>[4x]VPEITTAQTIANSVVDAKKFDYLFGKATGNSHTLDRTNQLALEMKRLGVADDINGHAVLAEHFTQATKDSN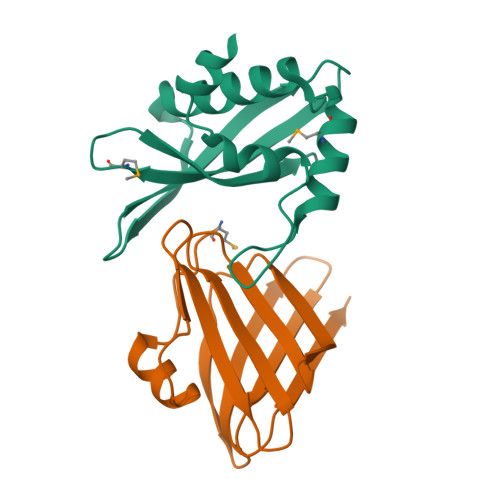NIVKKYTDQYGSFEIRESFFIGPSGKATVFESTFEVMKDGSHRFITTIPKNGVTK;>MFIENKPGEIELLSFFESEPVSFERDNISFLYTAKNKCGLSVDFSFSVVEGWIQYTVRLHENEILHNSIDGVSSFSIRNDNLGDYIYAEIITKELINKIEIRIRPDIKIKSSSVIR[4x]> SNVQTSADRVPHDLSHLVFEAGKIGRLKTISWTPVVAGDSFECDMVGAIRLSPLRRGLAVDSRVDIFSFYIPHRHIYGQQWINFMKDGVNASPLPPVTCSSGWDSAAYLGTIPSSTLKVPKFLHQGYLNIYNNYFKPPWSDDLTYANPSNMPSEDYKWGVRVANLKSIWTAPLPPDTRTSENMTTGTSTIDIMGLQAAYAKLHTEQERDYFMTRYRDIMKEFGGHTSYDGDNRPLLLMRSEFWASGYDVDG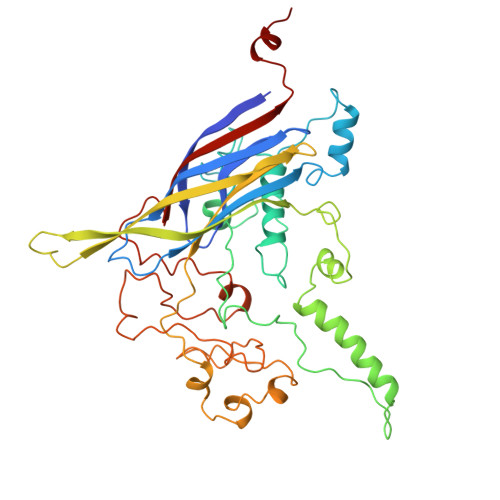TDQSSLGQFSGRVQQTFNHKVPRFYVPEHGVIMTLAVTRFPPTHEMEMHYLVGKENLTYTDIACDPALMANLPPREVSLKEFFHSSPDSAKFKIAEGQWYRTQPDRVAFPYNALDGFPFYSALPSTDLKDRVLVNTNNYDEIFQSMQLAHWNMQTKFNINVYRHMPTTRDSIMTS2-[(4-fluorophenyl)methyl]-2-azatricyclo[7.3.0.0^{3,7}]dodeca-1(9),3(7)-dien-8-imine 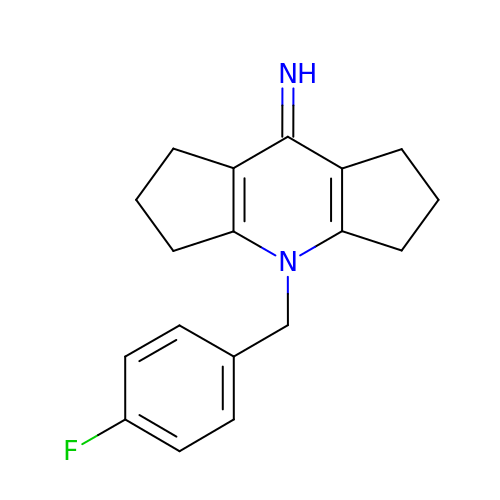| C18 H19 F N2 | DTKPOBDBQAIYNS-UHFFFAOYSA-N>[6x]MRVRTERLTLAGLSVLARIPEAPKALLLALHGLQGSKEHILALLPGY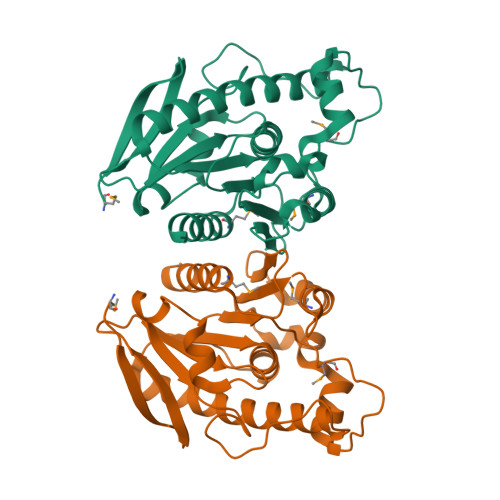AERGFLLLAFDAPRHGEREGPPPSSKSPRYVEEVYRVALGFKEEARRVAEEAERRFGLPLFLAGGSLGAFVAHLLLAEGFRPRGVLAFIGSGFPMKLPQGQVVEDPGVLALYQAPPATRGEAYGGVPLLHLHGSRDHIVPLARMEKTLEALRPHYPEGRLARFVEEGAGHTLTPLMARVGLAFLEHWLEAR>[4x]TKTESSSRGPYHPSECCFTYTTYKIPR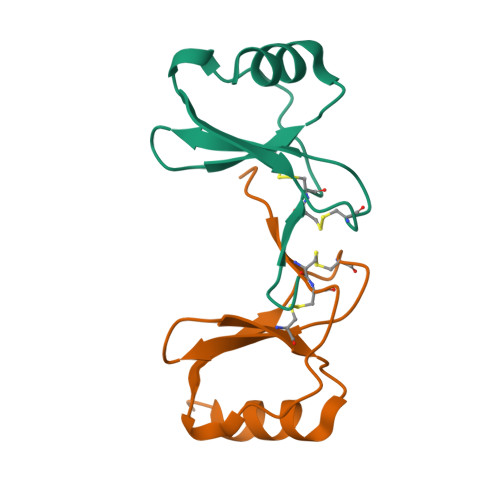QRIMDYYETNSQCSKPGIVFITKRGHSVCTNPSDKWVQDYIKDMKEN>[2x]GSHMAASITAITVENLEYPAVVTSPVTGKSYFLGG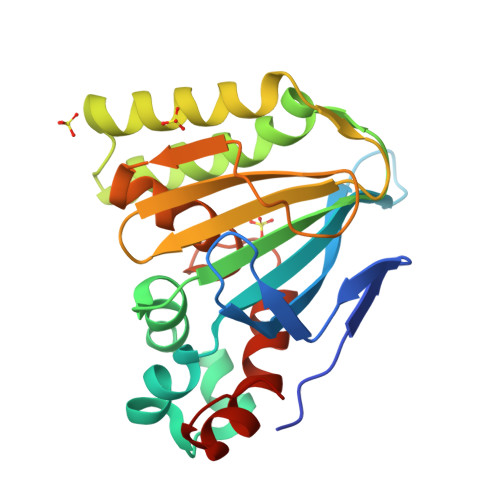AGERGLTIEGNFIKFTAIGVYLEDIAVASLAAKWKGKSSEELLETLDFYRDIISGPFEKLIRTSKIRELSGPEYSRKVMENCVAHLKSVGTYGDAEAEAMQKFAEAFKPVNFPPGASVFYRQSPDGILGLSFSPDTSIPEKEAALIENKAVSSAVLETMIGEHAVSPDLKRCLAARLPALLNEGAFKIGN> EFYTAPSTESKFTEVLSKAKLQYPTSTTVAFADDLLDGYAASYFYLTSDLYMQFQVAGSSQRSELREMETSGDEAAWDCTGSTAHVASAQIAIPVQE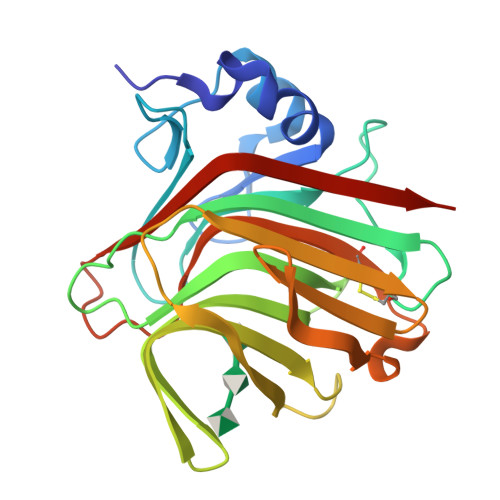DGIEEVTILQVHDSDVTPVLRISWVSSITIDGVTSEDVVLATIRNGIDDSTATKTVLQAHTTSRTEFNINVQNSKLSITVDGTTELDEADISQFDGSTCYFKAGAFNNNPTDTSANARIKMYELEWVDHHHHHH> ANKRMKVKHDDHYELIVDGRVYYICIVCKRSYVCLTSLRRHFNIHSWEKKYPCRYCEKVFPLAEYRTKHEIHHTGERRYQCLACGKSFINYQFMSSHIKSVHSQDPSGDSKLYRLHPCRSLQI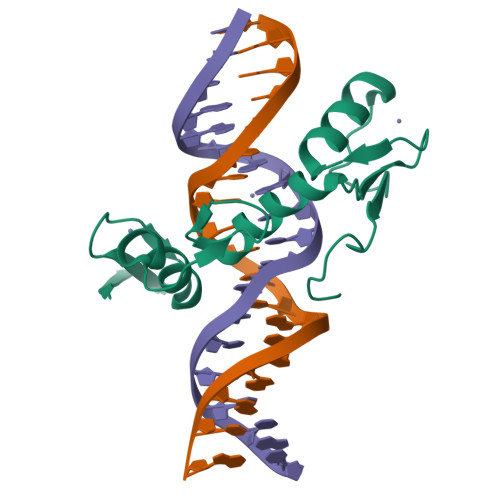RQYAYLSDRS> MGAGEKGIVEKEGYQLDTRRQAQAAYPRIKVLVIHYTADDFDSSLATLTDKQVSSHYLVPAVPPRYNGKPRIWQLVPEQELAWHAGISAWRGATRLNDTSIGIELENRGWQKSAGVKYFAPFEPAQIQALIPLAKDIIARYHIKPENVVAHADIAPQRKDDPGPLFPWQQLAQQGIGAWPDAQRVNFYLAGRAPHTPVDTASLLELLARYGYDVKPDMTPREQRRVIMAFQMHFRPTLYNGEADAETQAIA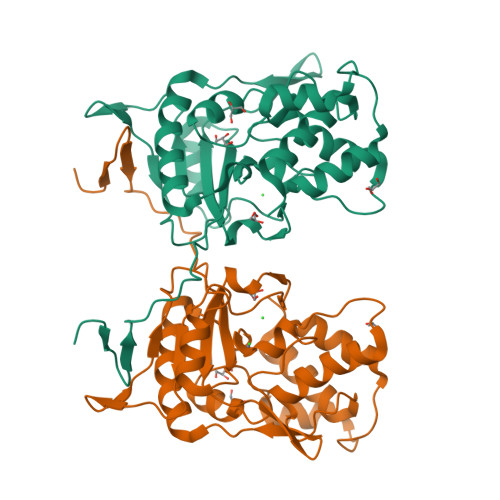EALLEKYGQD> GPGSMSIPTLNPTVALVAIDLQNGIVVLPMVPQSGGDVVAKTAELANAFRARKLPVIFVHTSYQPDGAVALKVKTDVPPSPPNLDPEWSAFAPALGVQPLDVVVTKHQWGAFTGTDLDVQ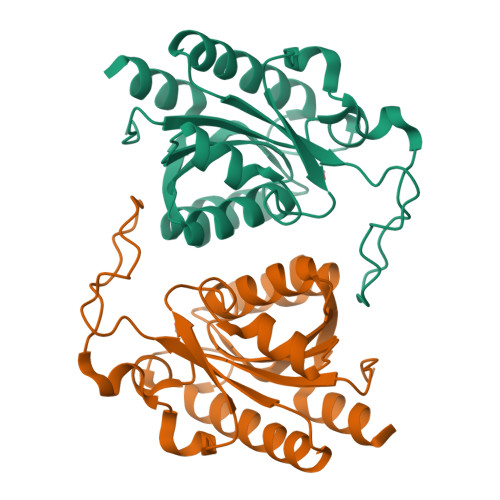LRRRGITDIVLTGIATNIGVESTAREAYENNYNVVVVSDAVSTWSTDAQTFALTQIFPKLGQVATAADVEAALETQQTR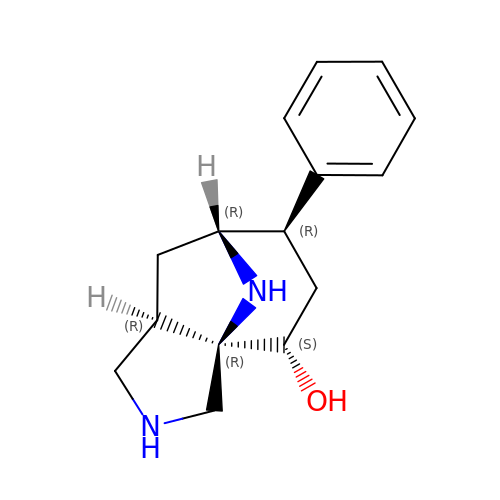(3aR,4S,6R,7R,8aR)-6-phenyloctahydro-1H-3a,7-epiminocyclohepta[c]pyrrol-4-ol | C15 H20 N2 O | WNBPFOXFPIFLPO-ZSAUSMIDSA-N> XXXXXXXTGLSEMRLEKDRFSVNLDVKHFSPEELKVKVLGDVIEVHGKHEERQDEHGFISREFHRKYRIPADVDPLTITSSLSSDG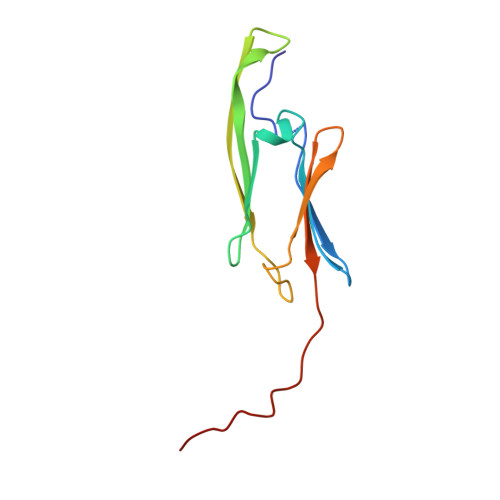VLTVNGPRKQVSGPERTIPITR> MAPGCKTELRSVTNGQSNQPSNEGDAIKVFVRIRPPAERSGSADGEQNLCLSVLSSTSLRLHSNPEPKTFTFDHVADVDTTQESVFATVAKSIVESCMSGYNGTIFAYGQTGSGKTFTMMGPSESDNFSHNLRGVIPRSFEYLFSLIDREKEKAGAGKSFLCKCSFIEIYNEQIYDLLDSASAGLYLREHIKKGVFVVGAVEQVVTSAAEAYQVLSGGWRNRRVASTSMNRESSRSHAVFTITIESMEKSNEIVNIRTSLLNLVDLAGSERQKDTHAEGMRLKEAGN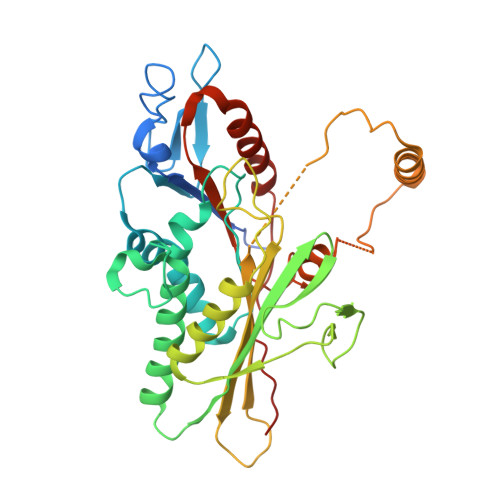INRSLSCLGQVITALVDVGNGKQRHVCYRDSKLTFLLRDSLGGNAKTAIIANVHPGSRCFGETLSTLNFAQRAKLIKNKAVVNEDTQG> IVGGYTCGANTVPYQVSLNSGYHFCGGSLINSQWVVSAAHCYKSGIQVRLGEDNINVVEGNEQFISASKSIVHPSYNSNTLNNDIMLIKLKSAASLNSRVASISLPTSCASAGTQCL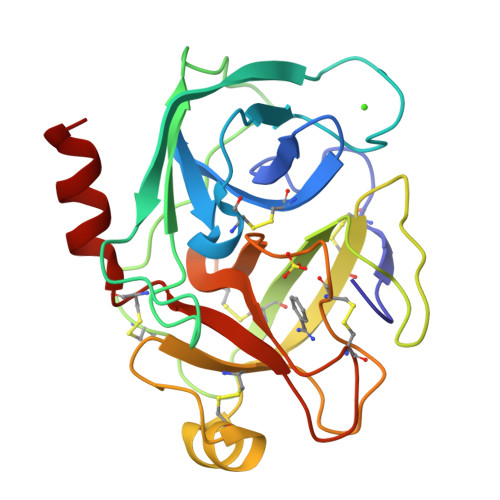ISGWGNTKSSGTSYPDVLKCLKAPILSDSSCKSASSRIITSNMFCAGYLEGGKDSCQGDSGGPVVCSGKLQGIVSWGSGCAQKNKPGVYTKVCNYVSWIKQTIASN> VDKVDYEIDYSTAGYSFWNEVNEEVKETTTIGKNDTEGCLEIKTSVAASQNHFIQYHTADNLPIEIGKEYKLKMMVRGSAEGKLNFGVGPWSGRAEGSFSFNTEWKEYEFSFKAVADGGHVMTQSGLFVG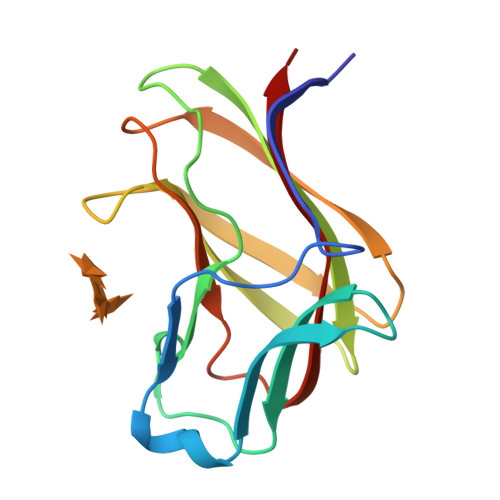TIQIKYVKITHS> MAQKPQRPRRPASPISTIQPKANFDAQQFAGTWLLVAVGSACRFLQEQGHRAEATTLHVAPQGTAMAVSTFRKLDGICWQVRQLYGD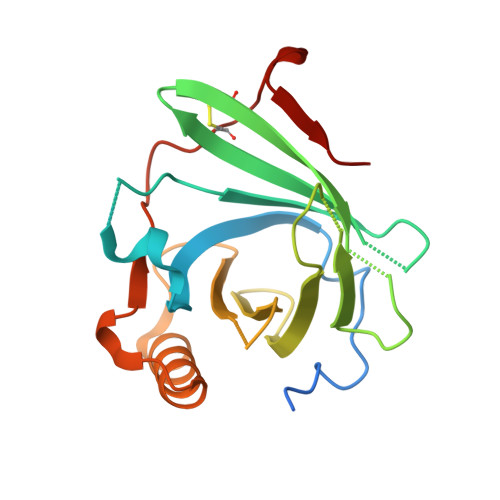TGVLGRFLLQARDARGAVHVVVAETDYQSFAVLYLERAGQLSVKLYARSLPVSDSVLSGFEQRVQEAHLTEDQIFYFPKYGFCEAADQFHVLDEVRR Here, we show that the Ty1 retrotransposon Copia forms virus-like capsids in vivo and transfers between cells. Copia is enriched at the Drosophila neuromuscular junction (NMJ) and transported across synapses, and disrupting its expression promotes both synapse development and structural synaptic plasticity. Because Copia behaves in a viral-like manner, we used cryogenic-electron microscopy (cryo-EM) to determine the high-resolution structure of the Copia capsid and found that it is distinct from the related dArc1 capsid, with a larger internal capacity and the presence of pores similar to those used by retroviruses to carry out their reverse transcriptase activity. The capsid layer is composed of the Copiagag protein’s CA region, which contains 2 alpha-helical domains.

To enhance the resolution of the capsid region, we used local reconstruction methods to determine the structures of individual subregions of capsid known as capsomers, which are sub-assemblies that are found at the vertices or faces of the icosahedron. Local reconstruction of the pentameric capsomers found at the vertices provided a map to an overall resolution of ~3.3-Å. The high-quality maps of the locally refined capsomers allowed us to build an atomic model of the Copiagag protein with high confidence and good stereochemistry. The NTDs form central spokes at the center of each capsomer sub-assembly, while the CTD is arranged in the capsomer periphery. In place of the spikes, the Copia capsid contains positively charged pores at the center of each hexameric or pentameric sub-assembly, similar to HIV. The positively charged pores of HIV function as gates for dNTP entry into the capsid for fueling reverse transcriptase activity. We hypothesize that the pores in the Copia capsid play a similar role. Despite the less extensive interfaces between capsid subunits in Copia, we observed an interesting interaction between adjacent CTDs that is not found in other retroelement-derived capsids. We suspect this CTD-CTD interaction plays a key role in stabilizing Copia capsids by locking down the periphery of each capsomer sub-assembly.

>MDKAKRNIKPFDGEKYAIWKFRIRALLAEQDVLKVVDGLMPNEVDDSWKKAERCAKSTIIEYLSDSFLNFATSDITARQILENLDAVYERKSLASQLALRKRLLSLKLSSEMSLLSHFHIFDELISELLAAGAKIEEMDKISHLLITLPSCYDGIITAIETLSEENLTLAFVKNRLLDQEIKIKNDHNDTSKKVMNAIVHNNNNTYKNNLFKNRVTKPKKIFKGNSKYKVKCHHCGREGHIKKDCFHYKRILNNKNKENEKQVQTATSHG[5x]> SMALGPFPAMENQVLVIRIKIPNSGAVDWTVH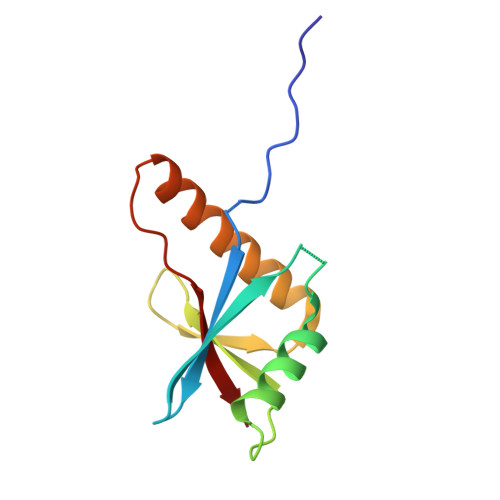SGPQLLFRDVLDVIGQVLPEATTTAFEYEDEDGDRITVRSDEEMKAMLSYYYSTVMEQQVNGQLIEPLQIFPRA> PISPIETVPVKLKPGMDGPKVKQWPLTEEKIKALVEICTEMEKEGKISKIGPENPYNTPVFAIKKKDSTKWRKLVDFRELNKRTQDFWEVQLGIPHPAGLKKNKSVTVLDVGDAYFSVPLDEDFRKYTAFTIPSINNETPGIRYQYNVLPQGWKGSPAIFQSSMTKILEPFKKQNPDIVICQYMDDLYVGSDLEIGQHRTKIEELRQHLLRWGLTTPDKKHQKEPPFLWMGYELHPDKWTVQPIVLPEKDSWTVNDIQKLVGKLNWASQIYPGIKVRQLCKLLRGTKALTEVIPLTEEAELELAENREILKEPVHGVYYDPSKDLIAEIQKQGQGQWTYQIYQEPFKNLKTGKYARMRGAHTNDVKQLTEAVQKITTESIVIWGKTPKFKLPIQKETWETWWTEYWQATWIPEWEFVNTPPLVKLWYQLEKEPIVGAETFYVDGAANRETKLGKAGYVTNKGRQKVVPLTNTTNQKTELQAIYLALQDSGLEVNIVTDSQYALGIIQAQPDKS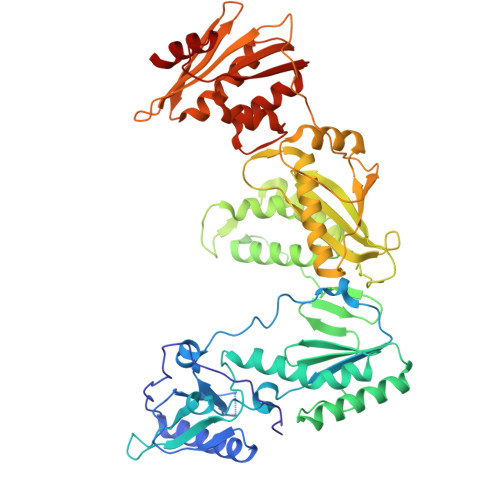ESELVNQIIEQLIKKEKVYLAWVPAHKGIGGNEQVDKLVSAGIR> MNHKVHHHHHHIEGRHMPLNNYLHVFYYSWYGNPQFDGKYIHWNHPVLEHWDPRIAKNYPQGRHNPPDDIGSSFYPELGSYSSRDPSVIETHMRQMRSASIGVLALSWYPPDVNDENGEPTDNLVPTILDKAHKYNLKVTFHIEPYSNRDDQNMYKNVKYIIDKYGNHPAFYRYKTKTGNALPMFYVYDSYITKPEKWANLLTTSGSRSIRNSPYDGLFIALLVEEKHKYDILQSGFDGIYTYFATNGFTYGSSHQNWASLKL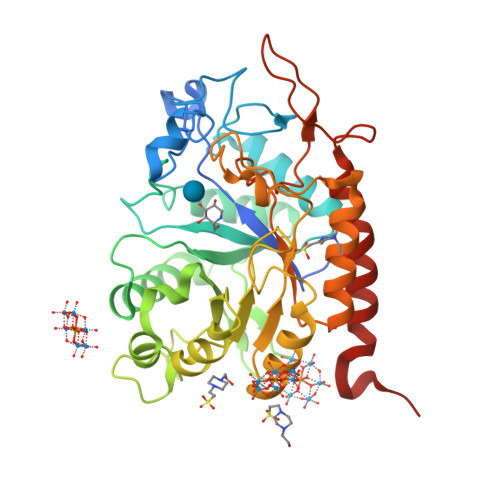FCDKYNLIFIPSVGPGYIDTSIRPWNTQNTRNRINGKYYEIGLSAALQTRPSLISITSFNEWHEGTQIEKAVPKRTSNTVYLDYRPHKPGLYLELTRKWSEKYSKERATYALDRQLPVS>MDLRDIDLNLLVVFNQLLLDRSVSTAGEKLGLTQPAVSNSLKRLRTALNDDLFLRTSKGMEPTPYALHLAEPVIYALNTLQTALTTRDSFDPFASTRTFNLAMTDIGEMYFMPPLMEALAQRAPHIQISTLRPNAGNLKEDMESGAVDLALGLLPELQTGFFQRRLFRTRYVCMFRKDHPSAKSPMSLKQFSELEHVGVVALNTGHGEVDGLLERAGIKRRMRLVVPHFIAIGPILHSTDLIATVPQRFAVRCEVPFGLTTSPHPAKLPDIAINLFWHAKYNRDPGNMWLRQLFVELFSEARHHHHHH[2x]

of transcription factors found in prokaryotes. N-terminal winged Helix Turn Helix (wHTH) DNA Binding Domain (DBD). two Rossmann fold-like sub domains (RD1, RD2). conformational changes which modify LTTR DNA binding sites promoter region DNA.

configuration formed by the association of two symmetry-related dimers. apo-DntR above, the conformations of their IBCs to be very similar. suggested, acting as mimics of bound salicylate.>[3x]MTKRVRLSDSFNPVYPYEDESTSQHPFINPGFISPNGFTQSPNGVLTLKCLTPLTTTGGSLQLKVGGGLTVDDTNGFLKENISATTPLVKTGHSIGLPLGAGLGTNENKLCIKLGQGLTFNSNNICIDDNINTLWTGVNPTEANCQIMNSSESNDCKLILTLVKTGALVTAFVYVIGVSNNFNMLTTHRNINFTAELFFDSTGNLLTRLSSLKTPLNHKSGQNMATGAITNAKGFMPSTTAYPFNDNSREKENYIYGTCYYTASDRTAFPIDISVMLNRRAINDETSYCIRITWSWNTGDAPEVQTSATTLVTSPFTFYYIREDD;> MARSPGRAYALLLLLICFNVGSGLHLQVLSTRNENKLLPKHPHLVRQKRAWITAPVALREGEDLSKKNPIAKIHSDLAEERGLKITYKYTGKGITEPPFGIFVFNKDTGELNVTSILDREETPFFLLTGYALDARGNNVEKPLELRIKVLDINDNEPVFTQDVFVGSVEELSAAHTLVMKINATDADEPNTLNSKISYRIVSLEPAYPPVFYLNKDTGEIYTTSVTLDREEHSSYTLTVEARDGNGEVTDKPVKQAQVQIRILDVNDNIPVVENKVLEGMVEENQVNVEVTRIKVFDADEIGSDNWLANFTFASGNEGGYFHIETDAQTNEGIVTLIKEVDYEEMKNLDFSVIVANKAAFHKSIRSKYKPTPIPIKVKVKNVKEGIHFKSSVISIYVSESMDRSSKGQIIGNFQAFDEDTGLPAHARYVKLEDRDNWISVDSVTSEIKLAKLPDFESRYVQNGTYTVKIVAISEDYPRKTITGTVLINVEDINDNCPTLIEPVQTICHDAEYVNVTAEDLDGHPNSGPFSFSVIDKPPGMAEKWKIARQESTSVLLQQSEKKLGRSEIQFLISDNQGFSCPEKQVLTLTVCECLHGSGCREAQHDSYVGLGPAAIALMILAFLLLLLVPLLLLMCHCGKGAKGFTPIPGTIEMLHPWNNEGAPPEDKVVPSFLPVDQGGSLVGRNGVGGMAKEATMKGSSSASIVKGQHEMSEMDGRWEEHRSLLSGRATQFTGATGAIMTTETTKTARATGASRDMAGAQAAAVALNEEFLRNYFTDKAASYTEEDENHTAKDCLLVYSQEETESLNASIGCCSFIEGELDDRFLDDLGLKFKTLAEVCLGQKIDINKEIEQRQKPATETSMNTASHSLCEQTMVNSENTYSSGSSFPVPKSLQEANAEKVTQEIVTERSVSSRQAQKVATPLPDPMASRNVIATETSYVTGSTMPPTTVILGPSQPQSLIVTERVYAPASTLVDQPYANEGTVVVTERVIQPHGGGSNPLEGTQHLQDVPYVMVRERESFLAPSSGVQPTLAMPNIAVGQNVTVTERVLAPASTLQSSYQIPTENSMTARNTTVSGAGVPGPLPDFGLEESGHSNSTITTSSTRVTKHSTVQHSYS;> MEPPGRRECPFPSWRFPGLLLAAMVLLLYSFSDACEEPPTFEAMELIGKPKPYYEIGERVDYKCKKGYFYIPPLATHTICDRNHTWLPVSDDACYRETCPYIRDPLNGQAVPANGTYEFGYQMHFICNEGYYLIGEEILYCELKGSVAIWSGKPPICEKVLCTPPPKIKNGKHTFSEVEVFEYLDAVTYSCDPAPGPDPFSLIGESTIYCGDNSVWSRAAPECKVVKCRFPVVENGKQISGFGKKFYYKATVMFECDKGFYLDGSDTIVCDSNSTWDPPVPKCLKVLPPSSTKPPALSHSVSTSSTTKSPASSASGPRPTYKPPVSNYPGYPKPEEGILDSLDVWVIAVIVIAIVVGVAVICVVPYRYLQRRKKKGTYLTDETHREVKFTSL

Among human species B adenovirus, HAdV-11, has the particular feature of exploiting two primary receptors, desmoglein 2 (DSG2) and CD46, to mediate cell attachment. Interactions between HAdV-11 and CD46 are well-characterized and clearly depend on the fiber protein, but the mechanism whereby HAdV-11 engages DSG2 has been still unresolved. In this study, we elucidate the molecular basis for HAdV-11 recognition of DSG2 by resolving the structure of extracellular domains of DSG2 in complex with the HAdV-11 fiber knob protein. The structure shows that DSG2 and CD46 engage different HAdV-11 residues and interfaces without overlapping.

By playing with the stoichiometry of the two receptors, we successfully obtained a “super-complex” composed of the HAd11K trimeric fiber knob with only one molecule of DSG2 and only one molecule of CD46. A large data set of HAd11K/rDSG2/rCD46 was acquired by cryo-EM, and the image analysis shows that there was a mixture of different complexes in solution even though the molecular ratio of rDSG2 to rCD46 was optimized to produce a ternary complex. Indeed, populations composed of rDSG2 and rCD46 alone were detected along with a “super complex” of HAd11K interacting with one rDSG2 and one rCD46 molecule. As both rDSG2 and rCD46 bind with two different monomers of HAd11K, they have one interacting monomer in common. But as rDSG2 binds to the apex of the knob and rCD46 the periphery of it, they do not prevent each other from simultaneously attached to the trimeric knob. In the ternary complex, rDSG2 binds to HAd11K in a nearly identical way as when rCD46 is not included, and the details of the interaction are, therefore, not recapitulated here. In the super-complex, rCD46 binds to two different HAd11K monomers at the periphery of the knob in a very similar way as it has been reported in a previous crystal structure. Indeed, the HI and DG loops of one monomer make extensive contacts with the SCR1 and the SCR1-SCR2 interface and the IJ loop of the neighboring monomer interacts with the base of SCR2. Key residues for the rCD46/HAd11K interaction identified in the crystal structure are similarly important in the cryoEM structure such as the salt bridges and hydrogen bonds between H43 of rCD46/D284 of HAd11K and E63 of rCD46/R280 of HAd11K.(3~{S},4~{R},5~{R})-4,5-bis(oxidanyl)-1-propyl-piperidine-3-carboxylic acid 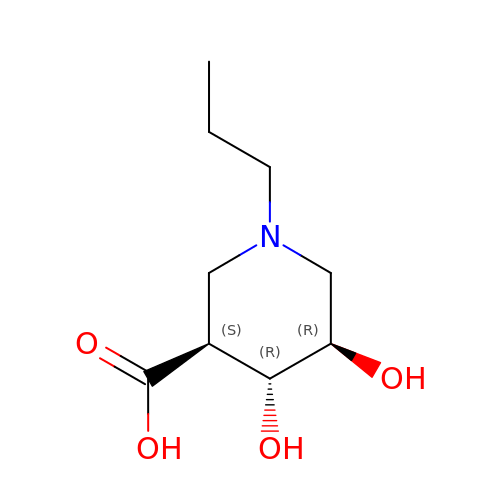| C9 H17 N O4 | RNWXBQBXRPVHBZ-XLPZGREQSA-N> KVFERCELARTLKRLGMDGYRGISLANWMCLAKWESGYNTRATNYNAGDRSTDYGVFQINSRYWCNDGKTPGAVNAAHLSCSALLQDNIAD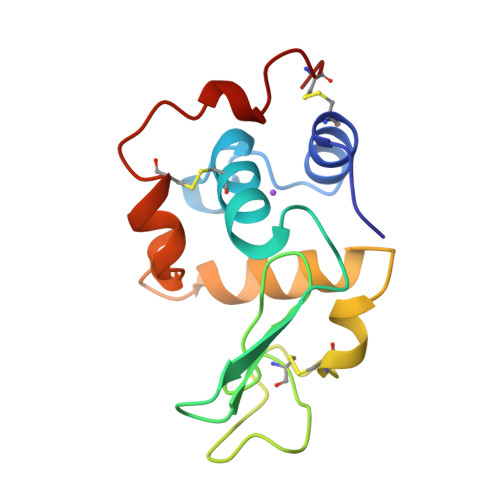AVAAAKRVVRDPQGIRAWVAWRNRCQNRDVRQYVQGCGV> MRGSHHHHHHGSMDRAAQIKQIADSWNTPRFAGIVRPYTPEDVYRLRGSVQIEYTLARMGAERLWNLLHTEPYINALGALTGNQAMQQVKAGLKAIYLSGWQVAADANLAGQMYPDQSLYPANSGPQLVRNINNALRRADQIYHSEGRNDIYWFAPIVADAEAGFGGPLNVFEIMKAYIE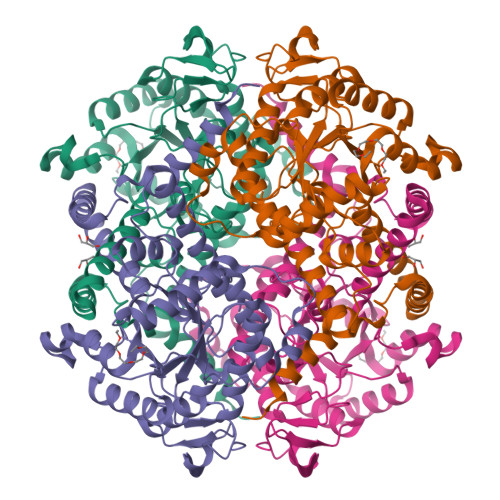AGAAGVHFEDQLASEKKCGHMGGKVLIPTQAAIRNLVAARLAADVMGVPTIIVARTDANAATLLTSDIDERDRPFCTGERTSEGFYRVRAGLDQAIARGLAYAPYADMIWCETSEPNLEEARRFAEAIHAQFPGKLLAYNCSPSFNWKKKLDDATIAAFQRELGAMGYKFQFVTLAGFHALNYSMFELARNYRDRGMAAYSELQQAEFAAEAYGYTATRHQREVGTGYFDEVAQVIAGGEISTTALTGSTEEEQFH1-(4-hydroxy-3-nitrophenyl)quinazoline-2,4(1H,3H)-dione 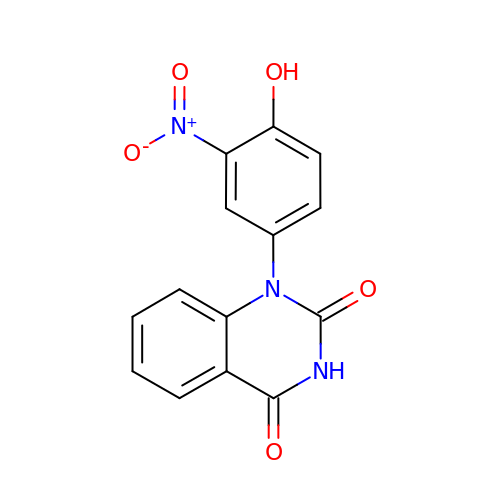| C14 H9 N3 O5 | YVQCKIRAVMSRGN-UHFFFAOYSA-N4-[6-({4-[(fluorosulfonyl)oxy]phenyl}ethynyl)-4,4-dimethyl-3,4-dihydroquinolin-1(2H)-yl]-4-oxobutanoic acid 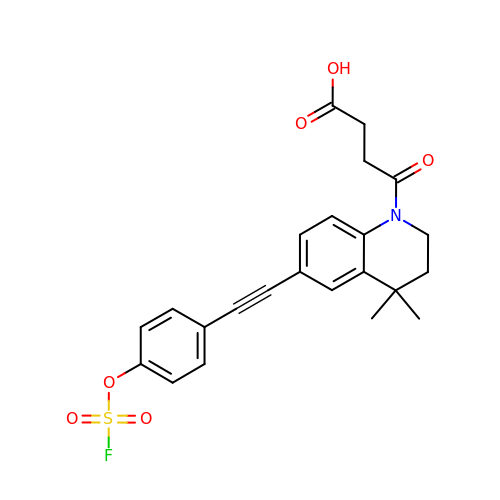| C23 H22 F N O6 S | OJLXEIKKMUTWLF-UHFFFAOYSA-N methyl 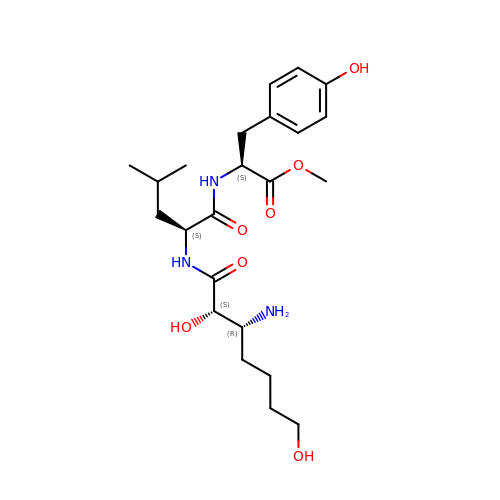(2~{S})-2-[[(2~{S})-2-[[(2~{S},3~{R})-3-azanyl-2,7-bis(oxidanyl)heptanoyl]amino]-4-methyl-pentanoyl]amino]-3-(4-hydroxyphenyl)propanoate | C23 H37 N3 O7 | LCFWQIPNOMDXPJ-FYQPLNBISA-N>MKDYKSITIATEGSYAPYNFKDAGGKLIGFDIDLGNDLCKRMNIECKFVEQAWDGIIPSLTAGRYDAIMAAMGIQPAREKVIAFSRPYLLTPNTFLTTADSPLLKTQVAIENLPLDNITPEQKAELDKFTKIFEGVKFGVQAGTSHEAFMKQMMPSVQISTYDTIDNVVMDLKAGRIDASLASVSFLKPLTDKPDNKDLKMFGPRMT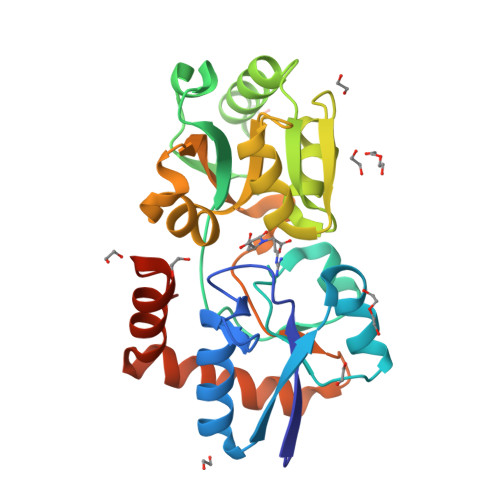GGLFGKGVGVGIRKEDADLKALFDKAIDAAIADGTVQKLSQQWFGYDASPKQHHHHHH[2x]>[4x]HHHHHHGSMNLTIIGSGSVGLVTGACLADIGHDVFCLDVDQAKIDILNNGGVPIHEPGLKEVIARNRSAGRLRFSTDIEAAVAHGDVQFIAVGTPPDEDGSADLQYVLAAARNIGRYMTGFKVIVDKSTVPVGTAERVRAAVAEELAKRGGDQMFSVVSNPE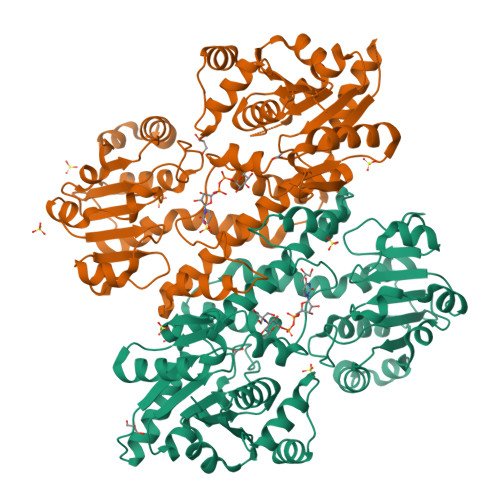FLKEGAAVDDFTRPDRIVIGCDDDVPGERARELMKKLYAPFNRNHERTLYMDVRSAEFTKYAANAMLATRISFMNELANLADRFGADIEAVRRGIGSDPRIGYHFLYAGCGYGGSCFPKDVEALIRTADEHGQSLQILKAVSSVNATQKRVLADKIVARFGEDLTGRTFAIWGLAFKPNTDDMREAPSRELIAELLSRGARIAAYDPVAQEEARRVIALDLADHPSWLERLSFVDDEAQAARDADALVIVTEWKIFKSPDFVALGRLWKTPVIFDGRNLYEPETMSEQGIEYHPIGRPGSRQAVAARVTGTAPASA>[2x]SNAMYKYITILGAAGQIAQKLTATLLTYTDMHITLYGR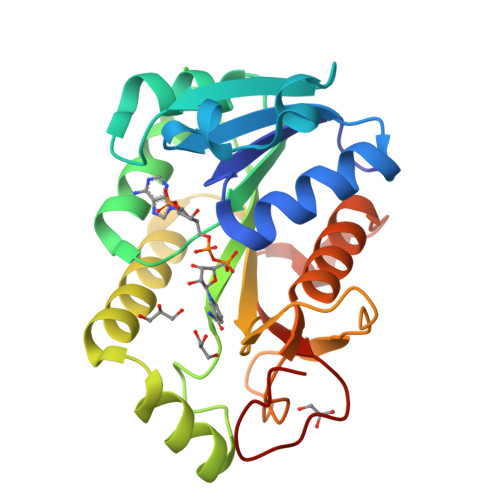QLKTRIPPEIIDHERVTVIEGSFQNPGKLEQAVTNAEVVFVGAMESGSDMASIVKALSRKNIRRVIGVSMAGLSGEFPVALEKWTFDNLPISYVQGERQARNVLRESNLNYTILRLTWLYNDPEKTDYELIPEGAQFNDAQVSREAVVKAIFDILHAADETPFHRTSIGVGEPGTHYDKPSFH>[4x]GMFASLIKRFQFVSVLDSNPQTKVMSLLGTIDNKDAIITAEKTHFLFDETVRRPSQDGRSTPVLYNCENEYSCINGIQELKEITSNDIYYWGLSVIKQDMESNPTAKLNLIWPATPIHIKKYEQQNFHLVRETPEMYKRIVQPYIEEMCNNGRLKWVNNILYEGAESERVVYKDFSEENKDDGFLILPDMKWDGMNLDSLYLVAIVYRTDIKTIRDLRYSDRQWLINLNNKIRSIVPGCYNYAVHPDELRILVHYQPSYYHFNIHIVNIKHPGLGNSIAAGKAILLEDIIEMLNYLGPEGYMNKTITYAIGENHDLWKRGLEEELTKQLERDGIPKIPKIVNGFK

In the 3′ to 5′ pathway, the mRNA body is processively hydrolyzed by the 10-component cytoplasmic exosome complex (exo-10; exo-9 plus Rrp44/Dis3), followed by the removal of the cap structure of the remaining short RNA fragment by the Scavenger Decapping enzyme DcpS (Dcs1p in yeast). The apo DcpS decapping enzyme assembles into an 80-kDa symmetric homodimer that contains dimeric N- and C-terminal domains that are linked by a flexible hinge region. The enzyme possesses two bipartite active sites that are located at the interface between the N- and C-terminal domains. Upon substrate binding to the C-terminal part of one of the active sites, the N-terminal domain flips over to enclose the mRNA substrate in a well-defined pocket.

To obtain insights into the mechanism that prevents DcpS from forming a productive active site around mRNA substrates longer than two nucleotides, we determined the crystal structure of DcpS in complex with a capped dinucleotide (note: DcpS contains the H268N inactivating mutation). The complex crystallized in space group P212121, with two dimers per asymmetric unit. The final model was refined to 2.9-Å resolution with good geometry. In this structure, DcpS is in the asymmetric conformation, with the N-terminal lid domain flipped over such that the substrate is tightly embeded in the closed active site. The methylated guanine cap structure is tightly embedded in the active site and stabilized by stacking interaction with Trp-161. Importantly, the structure also displays clear density for the mRNA body of the capped dinucleotide. This reveals the path of the mRNA inside the closed active site and shows that the RNA body has no sequence specific interaction within the binding site. The second nucleotide points away from the cap structure, toward a narrow opening between the N- and C-terminal domains and fully occupies this region of the active site. However, with a diameter of ∼7 Å, the channel is too small to accommodate a putative third nucleotide. This is confirmed by modeling of a capped trinucleotide into the closed active site, which shows that the van der Waals radii of a third nucleotide and residues of the exit channel significantly overlap.> PGGGWKVGDRANHRKWGIGTVVSVRGGG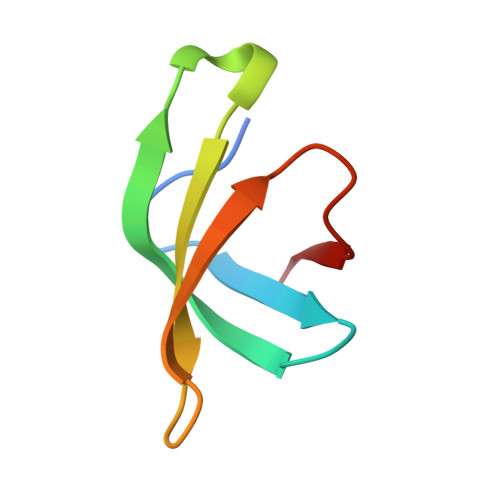DDQELDIAFPSPIGIKRLLAKFAPIEKV>MGYLHRVVEGLKANAGGEALVSADRRLTGAETLEEIHRTARALAAQGLRPGDGVVTLHGNGVEAVVLRIAVQLLGCRYAGLRPVFATREKANFLAEAEAAAFVYQPDMADEAAELLREVPTPRVLSLGPAPLGEDLVALAGAQSAEPVEFTADERAATAVGFTGGTTGRAKGVCRAPFDLEACLDASLTIFGEGPWRFLVCIPIADLGGEMAEWTLAAGGTVVLREDFEPADILATIGAERTTHVFCAPGWVYQLAEHPALADADLSSLTQIPYGGAPSTPARIADALEKLGRPLLVHCYGSQEGGWMTWLSAEDHVRADRYLLNSVGKALPGTEIAIRDQDGADLPVGTVGEVCVRSTMLMRGYWRLPELTAKTVRDGWLHTGDLGRLDTEGYLYLVDRAKDVIIVEAYNVYSQEVEHVLTGHPDVRYAAVVGVPDHDTTEAVYAAVVPAEGVGEIDVDELRALVRTTLGPVHEPKHLDVVDTIPTTPRGHPDKSALRTRWRAAQRA[2x]

Amide Bond Synthetases (ABSs) actively catalyze both the ATP-dependent adenylation of carboxylic acid substrates and their subsequent amidation using an amine nucleophile, both within the active site of the enzyme, enabling the use of only a small excess of the amine partner. In this report, we describe the activity and specificity of an ABS from Streptoalloteichus hindustanus (ShABS), with a broader, complementary substrate spectrum to that of McbA that includes enantioselective behavior toward an expanded range of acid and amine partners in amidation reactions. The requirement for large excesses of amine in these reactions has prompted investigations into the ATP-dependent amide bond synthetase (ABS) class of enzymes, also members of the larger ANL (acyl-CoA synthetase–non-ribosomal peptide synthase–luciferase) family of adenylase enzymes, as these catalyze both the formation of the adenylate and the amidation reaction within one active site of the enzyme and require only one or low equivalents of the amine as a coupling partner. In common with other adenylases, McbA features a larger N-terminal domain coupled to a C-terminal “cap” domain.

In order to explore the basis for the broader substrate specificity of ShABS, the three-dimensional structure was determined by using X-ray crystallography (SI Section 4). As crystals of wild-type ShABS were initially not forthcoming, two mutants, K492A and K492H, of a lysine residue K492 implicated in interacting with ATP were prepared and subjected to crystallization trials, in an attempt to obtain a structure. Although no crystals were obtained in the presence of ATP or AMP and acid substrate, the inclusion of the noncleavable ATP analogue α,β-methylene adenosine 5′-triphosphate (AMP-CPP) was successful in giving diffracting crystals of ShABS K492H in the P21 space group, from which were obtained data sets that were refined to 2.01 (Data set #1) and 2.57 Ångstrom (Data set #2) resolution, the second of which contained density for AMP-CPP in the active site. This structure of ShABS (ShABSAdFigure 1a) featured two molecules in the asymmetric unit cell, each of which corresponded to the “adenylation” conformation of McbA, with an rmsd between the two enzymes of 1.50 Å over 469 C-α atoms. The major differences in active site residues between the ShABSAd and McbAAd acid binding sites were W307 (ShABS) for F301 (McbA), W214 for C209, R175 for H170, C299 for N293, and S302 for T296. The presence of the two tryptophan residues is most likely to account for the differences in acid specificity between McbA and ShABS.The mucolytic human gut microbiota specialist Akkermansia muciniphila is proposed to boost mucin-secretion by the host, thereby being a key player in mucus turnover. Mucin glycan utilization requires the removal of protective caps, notably fucose and sialic acid, but the enzymatic details of this process remain largely unknown. Here, we describe the specificities of ten A. muciniphila glycoside hydrolases, which collectively remove all known sialyl and fucosyl mucin caps including those on double-sulfated epitopes. Structural analyses revealed an unprecedented fucosidase modular arrangement and explained the sialyl T-antigen specificity of a sialidase of a previously unknown family.

Although crystallization attempts of both AmGH29C/D were carried out, we could only determine the structure of AmGH29D, the most complex fucosidase structure to date. Unique to this structure is that the GBLD domain is joined to a linker domain and a C-terminal CBM32. The linker domain and the CBM32 adopt an extended conformation, which positions the CBM32 binding site above the catalytic domain. This juxtapositioning of the linker-CBM32 domain relative to the catalytic domain, which resembles a Cobra strike pose, is observed in the GH33 sialidase from Micromonospora viridifaciens, suggesting convergent evolution to a similar putative mucin-binding motif. The GBLD and the CBM32 assume the same fold, despite less than 22% shared sequence identity. The position and the surface chemistry of the putative binding sites of the GBLD and the CBM32 domains are different, suggesting their possible functional divergence. The catalytic site of AmGH29D is similar to the closest characterised counterpart from Streptococcus pneumonia, but differs by being flanked with a flat positively charged surface, compatible with binding sialylated or sulfated glycans at the mucin surface. Notably, shorter and more flexible loops result in a more open active site in AmGH29C as compared to AmGH29D. Notably, only AmGH29C, but not AmGH29D, showed activity on the double sulfated terminal Lex epitope highlighting the overall broader epitope specificity of AmGH29C.

>MNLNQLIKAAVLGGALCTACFAGAGPKGCLTPLKPVPSAEQLEWHDMEMYAFVHFTINTFTGKEWGYGDEKPELFHPSDFDADDLVRTLADAGFKGVVLTCKHHDGFCLWPTKTTLHSVAASPWKQGKGDVVKEVSRACGKYGVRFGVYLSPWDRNAASYGTPDYIRMYRQQLKELATGYGSIFLAWFDGANGGDGYYGGARERRSIDRSAYYDWKATWGELKKRQPGAVIFSDVGPDVRWVGNESGYAGYPCWATYTPVPLQAGTEPAPGTVRYRLGTEGTMDGKYWIPAEVDVSIRPGWFWHEHENSRVRTPENLLKLYFDSVGRGANLNLNVPPDRRGRIHEEDKKSLAGFRVLLDELYSRNFASGAQAESSSSWKGHGAEQVLDRKRTTYWVAAPEDKHPCVVLKLPEPAAFDVIRLAEPIQLGQRVRKFRVEVRENGQWSKWTEGASIGARVLLKGRPVTADGVRVVLEQSRAVPALCEVSLWKYPVILNAPAVNYDRNGRVTLASAENVVIRYTTDGTEPGPQSAMYRNPFFLPAGGTVKAAAEYRGRKSSVTTQIIPVPTRDWKVVAGERSAAAPELAIDGDSSTLWHTHAAQGELAPPQALEIDMGRPVNVAAVIYTPRRDSSTGTVDRYAVYLSMDGNTWGAPAAEGEFSNIRANPVPQRIDLKAPVKARYLRFVGKRVVEGSHVAVAELGVLGK[2x]>GEPDSLEVLVKTLDSQTRTFIV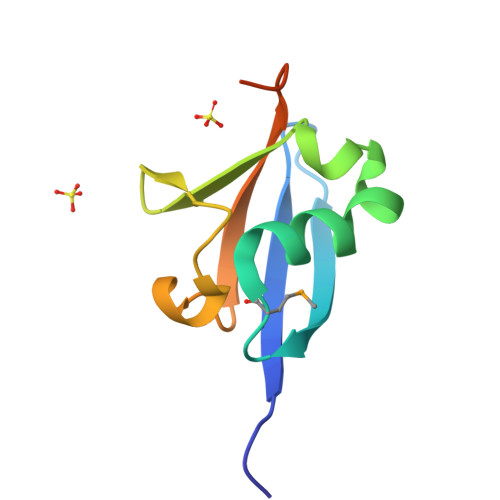GAQMNVKEFKEHIAASVSIPSEKQRLIYQGRVLQDDKKLQEYNVGGKVIHLVERAPPQTHLPSGASSG[2x]>[2x]GPALAQDDVAPYFKTEPGLPQIHLEGNRLVLTCLAEGSWPLEFKWIRNDSELTTYSSEYKYIIPSLQKLDAGFYRCVVRNRMGALLQRKSEIQVAYMGNFMDTDQRKTVSQGHAALLNLLPIVSCPQPQVTWFREGHKIIPSSRIAITLENQLVILATTASDAGAYYVQAVNEKNGENKTSPFIHLSVARDTGTHEAMAPIIVVAPGNRSVVAGSSETTLECIANARPVEELSVHWKRNGVRLT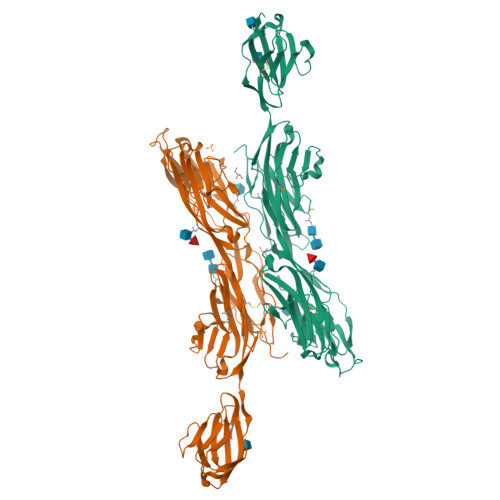SGLHSYGRRLTITNPTSADTGMYVCEATLRGSTFEPARARAFLSIIEPPYFTAEPESRILGEVEETMDIPCRAMGVPLPTLQWYKDAVPLSKLQNPRYKVLPSGGLHIQKLSPEDSGIFQCFASNEGGEVQTHTYLDVTNIAPAFTQRPVDTTVTDGMTAVLRCEVSGAPKPAITWKRGNHILASGSVRIPRFMLLESGGLRIAPVFIQDAGNYTCYAANTEASVNASAMLTVWNRT> MAEQFVGSGWSFPLRIGPTGGIALVSGEQEVEEAMRLILATAPGERPMRPEFGCAIHDLVFAPVNEQTAGRIQHEVYVTLDRWEPRIEVHDVDVTTGEEQNVLFIDVRYSIRGTNNPRSLVFPFYVIPSHDEPDLPDA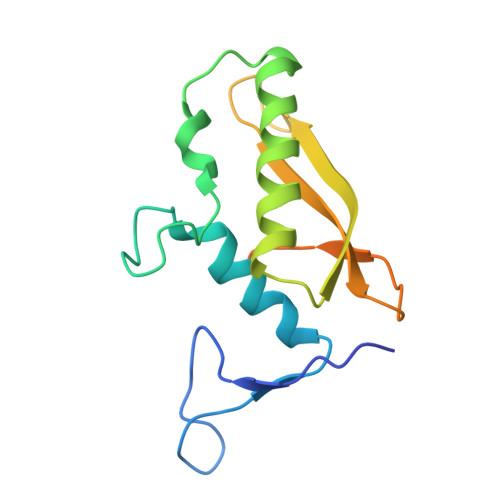PAGLPGSPESDR>MSSKPKPIEIIGAPFSKGQPRGGVEKGPAALRKAGLVEKLKETEYNVRDHGDLAFVDVPNDSPFQIVKNPRSVGKANEQLAAVVAETQKNGTISVVLGGDHSMAIGSISGHARVHPDLCVIWVDAHTDINTPLTASSGNLHGQPVAFLLKELKGKFPDVPGFSWVTPCISAKDIVYIGLRDVDPGEHYIIKTLGIKYFSMTEVDKLGIGKVMEETFSYLLGRKKRPIHLSFDVDGLDPVFTPATGTPVVGGLSYREGLYITEEIYKTGLLSGLDIMEVNPTLGKTPEEVTRTVNTAVALTLSCFGTKR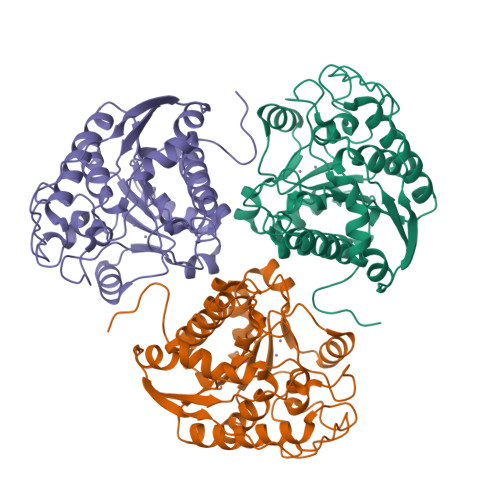EGNHKPETDYLKPPK[3x]>[24x]MSAEKKQNLQDTFLNSVRKSKTPLTIFLVNGVKL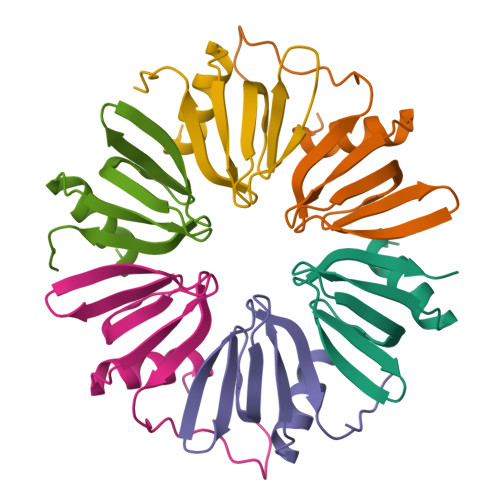QGVVSWFDNFCVLLRRDGQSQLVYKHAISTIMPAQPVQLYEPSADADD>KSCCPSTTGRNIYNTCRLTGSSRETCAKLSGCKIISASTCPSN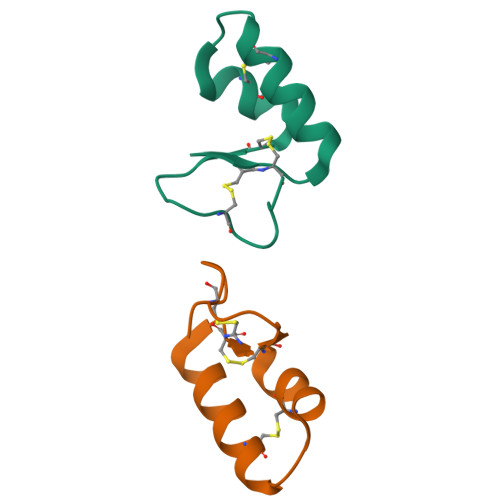YPK[2x]>[2x]MSAKKTNEKRSEIQSETNTTSLDEVAD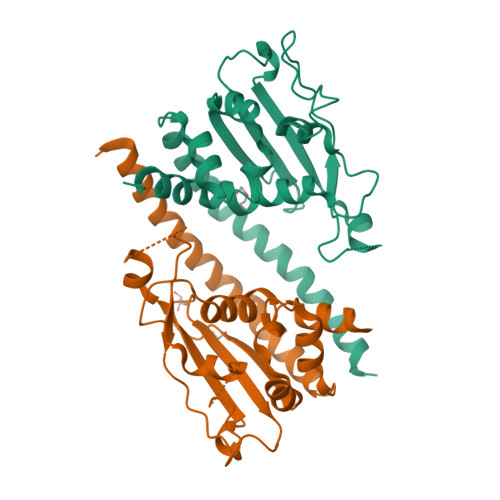IELEFEKADVELLKHQVELFNPLYEKRANVLRKIPKFWPIAIEAAPSDELSVYISPEDANVLEHLIDLRVYRPNEDPRDIKIVFEFEANEYLESNSLYLEKLFRYSSQKAEASSSNINKEPSQLISEKVNIEWKKNKDLTRQTKGTAPSFFTWFSWTGKENDIFEDEEELAIFIAEDLYPNAVKYFTDALQENEENEDEEIDLENENGDNISEEEPSKKRTKL> HMSLKSAVKTVLTNSLRSVADGGDWKVLVVDKPALRMISECARMSEILDLGVTVVEDVSKQRKVLPQFHGVYFIEPTEENLDYVIRDFADRTPTYEAAHLFFLSPVPDALMAKLASAKAVKYVKTLKEINTLFIPKEHRVFTLNEPHGLVQYYGSRSSSYNIDHLVRRLSTLCTTMNVAPIVRYSSTSTPGTERMAMQLQKEIDMSVSQGLINAREGKLKSQFLILDRAVDLKSPLVHELTYQAAAYDLLNIENDIYSYSTVDAGGREQQRQVVLGEDDDIWLQMRHLHISEVFRKVKSSFDEFCVSARRLQGLRDSQQGEGGAGALKQMLKDLPQHREQMQKYSLHLDMSNAINMAFSSTIDSCTKAEQNIVTEEEQDG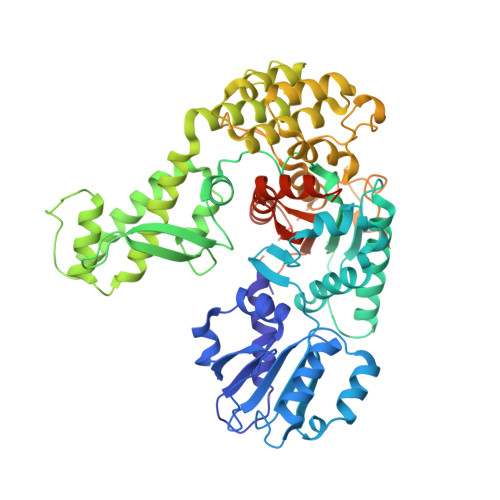NKVRDFIGEVASVVVDRRVSTEDKLRCLMLCVLAKNGTSSHELNNLLDNANIATPSRSAIYNLEMLGATVVADRRGRKPKTMKRIERDMPYVLSRWTPIVKDLMEYIATGQLDLESYPAVRDGPSVVQPKRASKSVEEDDDGPATSARKRGNWAKNKGNNRSLPSTPSGVAVSGNGAAGAAESAKPKLFVFINGTVSYNEIRCAYEVSQSSGYEVYIGAHNIATPAEFVELVSLLDKADQDVQVLTQGQGDGGLVITTGSAQAGLNLAEV> MERPESELIRQSWRVVSRSP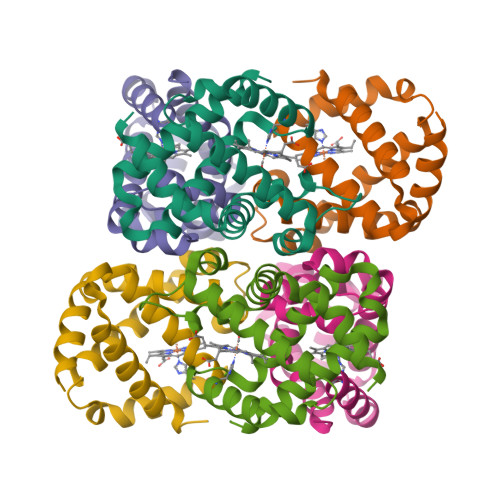LEHGTVLFARLFALEPSLLPLFQYNGRQFSSPEDSLSSPEFLDHIRKVMLVIDAAVTNVEDLSSLEEYLTSLGRKHRAVGVRLSSFSTVGESLLYMLEKSLGPDFTPATRTAWSRLYGAVVQAMSRGWDGE>QEQVAPPKDPAAALEDHKTRTDNRYEPSLDNLAQQDVAAPGAPEGVTALSDAQYNEANKIYFERCAGCHGVLRKGATGKALTPDLTRDLGFDYLQSFITYASPAGMPNWGTSGELSAEQVDLMANYLLLDPAAPPEFGMKEMRESWKVHVAPEDRPTQQENDWDLENLFSVTLRDAGQIALIDGSTYEIKTVLDTGYAVHISRLSASGRYLFVIGRDGKVNMIDLWMKEPTTVAEIKIGSEARSIETSKMEGWEDKYAIAGAYWPPQYVIMDGETLEPKKIQSTRGMTYDEQEYHPEPRV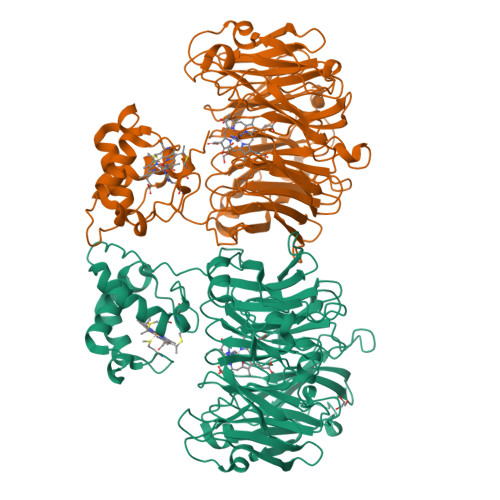AAILASHYRPEFIVNVKETGKILLVDYTDLNNLKTTEISAERFLHDGGLDGSHRYFITAANARNKLVVIDTKEGKLVAIEDTGGQTPHPGRGANFVHPTFGPVWATSHMGDDSVALIGTDPEGHPDNAWKILDSFPALGGGSLFIKTHPNSQYLYVDATLNPEAEISGSVAVFDIKAMTGDGSDPEFKTLPIAEWAGITEGQPRVVQGEFNKDGTEVWFSVWNGKDQESALVVVDDKTLELKHVIKDERLVTPTGKFNVYNTMTDTY[2x]> MTVTYTARVAKARFGGFSKLLLLWRGSIYKLLWRELLCFLGLFMALSAAYRFVLT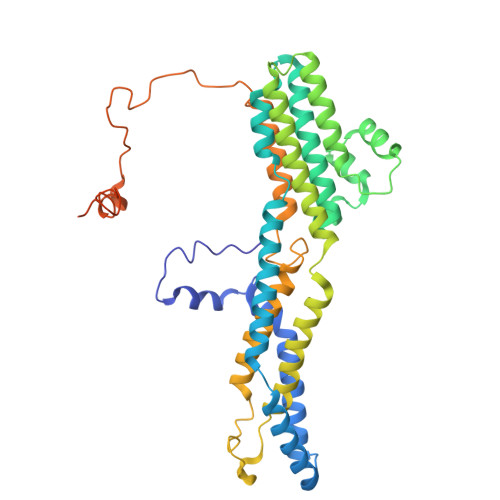EEQKRYFEKLVLYCDRYASLIPVSFVLGFYVTLVVHRWWNQYLSMPLTDALMCVVVGTVHGHDERGRLYRRTLMRYAGLSGVLILRSVSTAVFKRFPTIDHVVEAGFMTREERKKFENLNSSYNKYWVPCVWFCNLAAQARREGRIRDNGAFKLLLEELNVFRSKCGMLFHYDWISVPLVYTQVVTIAVYSYFLACLIGRQFLDPAQGYKDHDLDLCVPIFTLLQFFFYAGWLKVAEQLINPFGEDDDDFETNFLIDRCFQVSMLAVDEMYDDLAMLEKDLYWDAAEARAPYTAATAFLMQQPSFQGSTFDITLAKEDMQFQRQDGLEAPLNEAHGDFLQRLLPVGTGMGTGGLL>RSPWQGTLPPFLPCELQPHGLVNCNWLFLKSVPHFSAAAPRDNVTSLSLLSNRIHHLHDSDFAQLSNLQKLNLKWNCPPAGLSPMHFPCHMTIEPNTFLAVPTLEELNLSYNGITTVPALPSSLVSLILSRTNILQLDPTSLTGLHALRFLYMDGNCYYKNPCGRALEVAPGALLGLGNLTHLSLKYNNLTTVPRSLPPSLEYLLLSYNHIVTLAPEDLANLTALRVLDVGGNCRRCDHARNPCVECPHKFPQLHSDTFSHLSRLEGLVLKDSSLYQLNPRWFRGLGNLTVLDLSENFLYDCITKTKAFQGLAQLRRLNLSFNYHKKVSFAHLTLAPSFGSLLSLQELDMHGIFFRSLSQKTLQPLARLPMLQRLYLQMNFINQAQLGIFKDFPGLRYIDLSDNRISGAVEPVATTGEVDGGKKVWLTSRDLTPGPLDTPSSEDFMPSCKNLSFTLDLSRNNLVTVQPEMFAQLSRLQCLRLSHNSISQAVNGSQFVPLTSLQVLDLSHNKLDLYHGRSFTELPRLEALDLSYNSQPFSMRGVGHNLSFVAQLPTLRYLSLAHNGIHSRVSQQLCSTSLWALDFSGNSLSQMWAEGDLYLRFFQGLRSLIRLDLSQNRLHTLLPCTLGNLPKSLQLLRLRNNYLAFFNWSS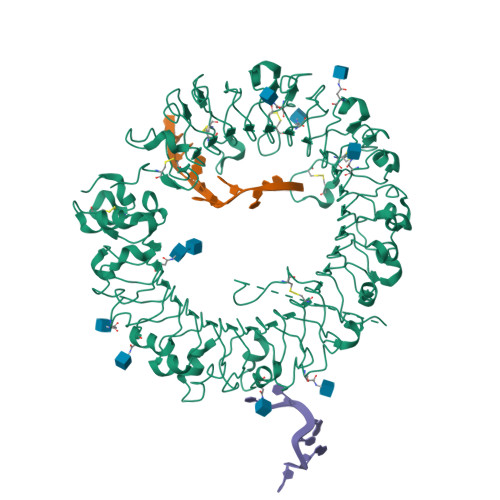LTLLPNLETLDLAGNQLKALSNGSLPSGTQLQRLDVSRNSIIFVVPGFFALATRLRELNLSANALRTVEPSWFGFLAGSLEVLDVSANPLHCACGAAFVDFLLQVQAAVPGLPSRVKCGSPGQLQGRSIFAQDLRLCLDESLSWDEFLVPR[2x]>TYCVAMHLADGLVFASDSRTNAGIDHIATFRKLFTFGTPGERLLVVQTAGNLATSQSVINLLQQRIRRDGASLLNVPSVYDATALVAETTREVMARDSGNLAGNTDLSCSFMVGGQIAGGPPALYSIYPQGNFIQATPDTPFLQLGESKYGKPILDRNLTFDTPLEQALRCALVSFDSTIRSNLSVGMPLDLLVYHRDSLILPEGYRVTEDDAYFSAIRRQWSAGLHDMLERLPSPPSAYNI[34x]

In 2008, a novel bacterial β subunit homolog, termed Anbu (ancestral β subunit) was identified. We find that Anbu forms a dodecameric open-ring assembly that locally resembles the architecture of the self-compartmentalizing proteasome, but is not closed for steric reasons. The individual subunits are essentially all in the same conformation, assuming the same fold as the proteasomal β subunit. Moreover, a comparison of the active sites shows the catalytic threonine and most other catalytically important residues in essentially the same conformation between Anbu, proteasomal β, and HslV, which suggests the same proteolytic mechanism for all three proteins. Via an extended C-terminal α-helical segment, Anbu forms a dimeric antiparallel coiled-coil interaction across this subunit interface, yielding a 3-fold increased interface area for this dimer compared with the respective subunits in the proteasome.

For experimental characterization, we recombinantly expressed the Anbu-1 protein from the pathogenic bacterium Pseudomonas aeruginosa (Pa-Anbu) in Escherichia coli. Crystallization trials yielded a monoclinic crystal form with large cell dimensions that led us to expect about three to four dozens of subunits per asymmetric unit. Unexpectedly, these 34 subunits in the asymmetric unit constitute the repeating unit of a continuous helix spanning the crystal. Within the helix, the subunits are arranged in 17 dimers of opposing protomers, distributed over two unequal helical turns. Consequently, the intra-dimer interface is virtually invariant and does not exceed 0.4 Å root-mean-square deviation (RMSD) in a superposition of all 17 dimers. This is contrasted by a high degree of variability in the lateral interface between the dimers, enabling the formation of the irregular helix with its two unequal turns that differ in the number of subunits and in the rise per turn: A superposition of all possible pairs of neighboring subunits yields RMSD values of up to 1.6 Å. We initially tried to fit the profile with modeled closed rings of six and seven Anbu dimers with different diameters, but could only obtain reasonable fits when using helical segments of six dimers from the Pa-Anbu crystal structure, clearly indicating that the solution structure is not a closed ring. However, the Pa-Anbu S1 pockets superimpose exceptionally well with those in the proteasome, revealing a relatively narrow, amphiphilic S1 pocket, in which F30 and L52 form a hydrophobic patch, whereas the moderately hydrophilic T20, T48, and S55 are oriented for hydrogen bonding to various positions in P1.> MQDLKNTKAPVSTATLNRNEFDSKTGNIYEAISIASKRAVQINSDIKKELLEKLEEFATYSDSLEEVFENKE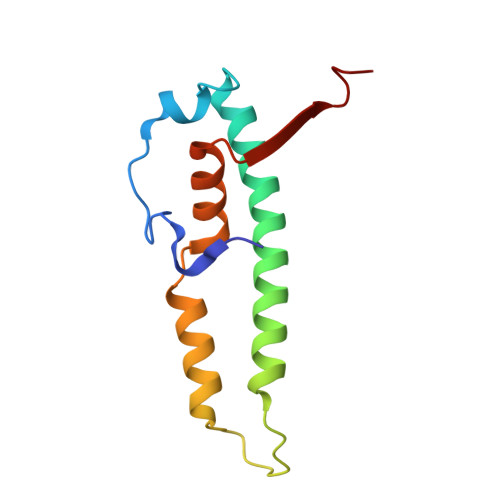QIEVSKFYEKLPKPHALAVQEWLEDKIYYRNTEKDA3,6,12,15,18,21,24-HEPTAOXAHEXATRIACONTAN-1-OL 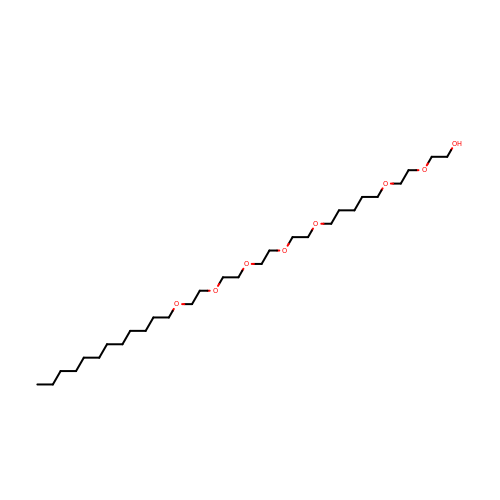| C29 H60 O8 | GEEFJAPPTAALTR-UHFFFAOYSA-N> MSFVAYEELIKEGDTAILSLGHGAMVAVRVQRGAQTQTRHGVLRHSVDLIGRPFGSKVTCGRGGWVYVLHPTPELWTLNLPHRTQILYSTDIALITMMLELRPGSVVCESGTGSGSVSHAIIRTIAPTGHLHTVEFHQQRAEKAREEFQEHRVGRWVTVRTQDVCRSGFGVSHVADAVFLDIPSPWEAVGHAWDALKVEGGRFCSFSPCIEQVQRTCQALAARGFSELSTLEVLPQVYNVRTVSLPPPDLGTGTDGPAGSDTSPFRSGTPMKEAVGHTGYLTFATKTPG;> MEGSGEQPGPQPQHPGDHRIRDGDFVVLKREDVFKAVQVQRRKKVTFEKQWFYLDNVIGHSYGTAFEVTSGGSLQPKKKREEPTAETKEAGTDNRNIVDDGKSQKLTQDDIKALKDKGIKGEEIVQQLIENSTTFRDKTEFAQDKYIKKKKKKYEAIITVVKPSTRILSIMYYAREPGKINHMRYDTLAQMLTLGNIRAGNKMIVMETCAGLVLGAMMERMGGFGSIIQLYPGGGPVRAATACFGFPKSFLSGLYEFPLNKVDSLLHGTFSAKMLSSEPKDSAL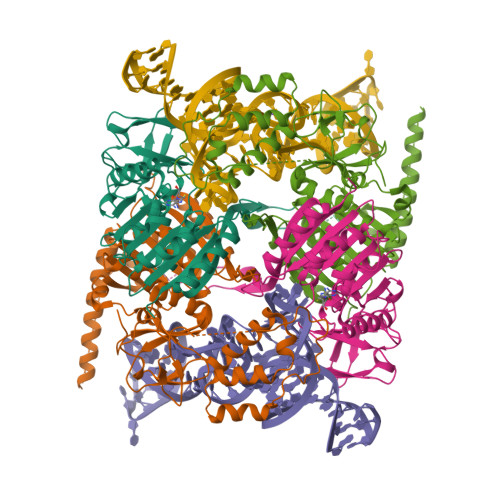VEESNGTLEEKQASEQENEDSMAEAPESNHPEDQETMETISQDPEHKGPKERGSKKDYIQEKQRRQEEQRKRHLEAAALLSERNADGLIVASRFHPTPLLLSLLDFVAPSRPFVVYCQYKEPLLECYTKLRERGGVINLRLSETWLRNYQVLPDRSHPKLLMSGGGGYLLSGFTVAMDNLKADTSLKSNASTLESHETEEPAAKKRKCPESDS> MEFAFYICGLIAILATLRVITHTNPVHALLYLIISLLAISGVFFSLGA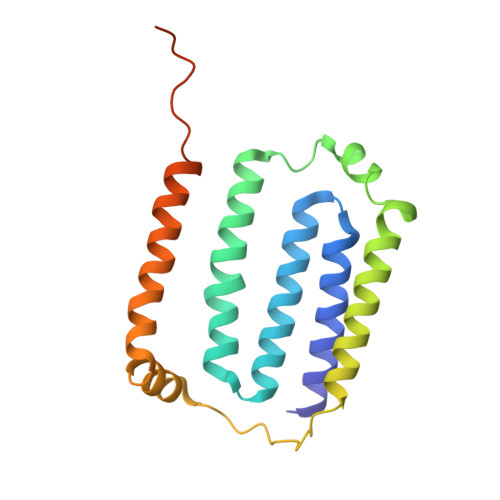YFAGALEIIVYAGAIMVLFVFVVMMLNLGGSEIEQERQWLKPQVWIGPAILSAIMLVVIVYAILGVNDQGIDGTPISAKAVGITLFGPYVLAVELASMLLLAGLVVAFHVGREERAGEVLSNRKDDSAKRKTEEHA>[2x]GMFLLQGAQMLQMLEKSLRKSLPMSLKVYGTVMHMNHGNPFNLKALVDKWPDFQTVVIRPQEQDMKDDLDHYTNTYHVYSEDLKNCQEFLDLPEVINWKQHLQIQSTQSSLNEVIQNLAATKSFKVKRSKNILYMASETIKELTPSLLDVKNLPVGDGKPKAIDPEMFKLSSVDPSHAAVV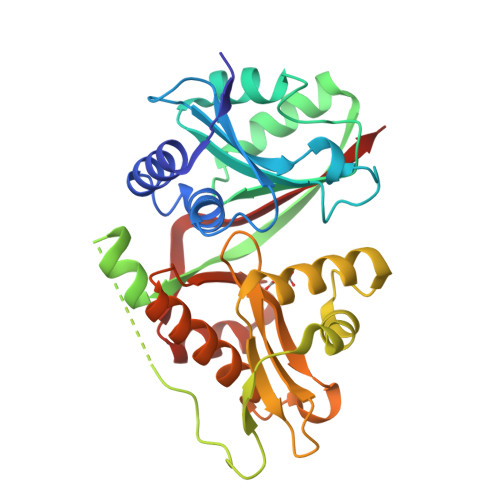NRFWLFGGNERSLRFIERCIQSFPNFCLLGPEGTPVSWSLMDQTGEMRMAGTLPEYRAQGLVTHAIYQQAQCLLKRGFPVYSHVDPKNQIMQKMSQSLNHVPMPSDWNQWNCEPL> GAMGMNSQKASKMTGSLKKNDLYIFDLSEQLLNSLKLMSFDNVMRCSVCQMSFDSRNEQKAHYQTDYHLMNVKRNLRGLDILSVEEFDALISKEHGIKSEDENSGGEQTSSDHEESEEASDRDPDLQTNNYMETIIENDLQKLGFQKDESDAISHINTQSPYIYFKSKYLQKNEVLAIYKSLFNKRSLSNPNEALTF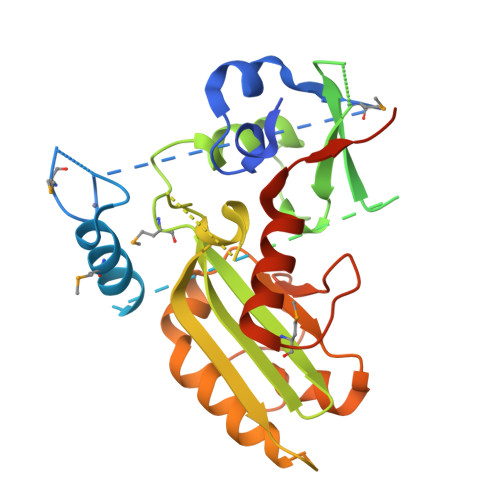WNSQENPMAISALFMVGGGHFAGAIVSHQRLNVKGNAHKKDETLIEQAVNFLEHKTFHRYTTRRKQGGSQSAMDNAKGKANSAGSALRRYNESALKTDIQGVLKDWEPYLSKCDNIFIRARNVSDKKIFTDNTVLNKGDERIKSFPFTTNRPTVLELKKAWCELSYLKILPKPEPLAVKETVQKLEVSNKKD>AFTGVERSTIGAIAKILASTPEAYGAEALARLFATHPGAKSYFDYAD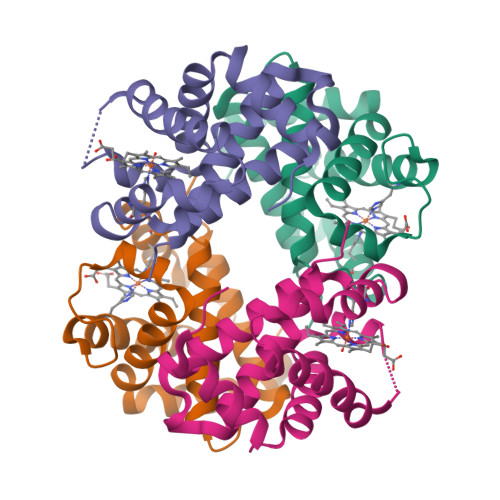YSAAGAKVQLHGGKVIRAVVSAAEHDDDLHAHLMVLAVTHGKKLLVDPSNFPMLSECILVTLATHLAEFSPATHCAVDKLLSAISSELSSKYR[2x];>[2x]VHWTQEERDEIVKTFFSANSSAIGTKALERMFVVFPWTNAYFAKXXXFSASIHAAIVVGALQDAVKHEDDVKAEFVNISKAHADKLHIDPGSFHLLTDSFIVELAHLKKVAFTPFVFAVWIKFFQVVIDAISSQYH>GHMSTLLINQPQYAWLKELGLREENEGVYNGSWGGRGEVITTYCPANNEPIARVRQASVADYEETVKKAREAWKIWADIPAPKRGEIVRQIGDALREKIQVLGSLVSLEMGKILVEGVGEVQEYVDICDYAVGLSRMIGGPILPSERSGHALIEQWNPVGLVGIITAFNFPVAVYGWNNAIAMICGNVCLWKGAPTTSLISVAVTKI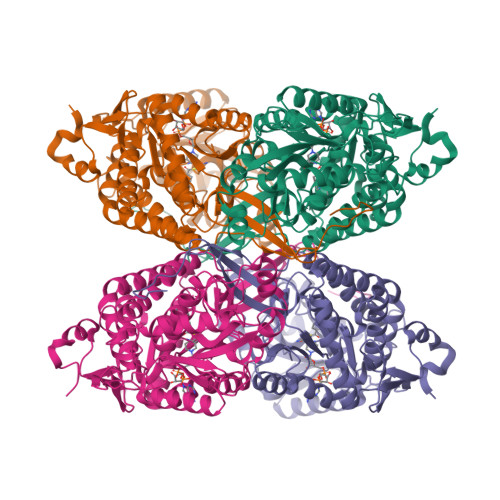IAKVLEDNKLPGAICSLTCGGADIGTAMAKDERVNLLSFTGSTQVGKQVGLMVQERFGRSLLELGGNNAIIAFEDADLSLVVPSALFAAVGTAGQRCTTARRLFIHESIHDEVVNRLKKAYAQIRVGNPWDPNVLYGPLHTKQAVSMFLGAVEEAKKEGGTVVYGGKVMDRPGNYVEPTIVTGLGHDASIAHTETFAPILYVFKFKNEEEVFAWNNEVKQGLSSSIFTKDLGRIFRWLGPKGSDCGIVNVNIPTSGAEIGGAFGGEKHTGGGRESGSDAWKQYMRRSTCTINYSKDLPLAQGIKFQ[4x]>MAMGQLQHGIDDENATKQTQKYRDAEQSKKTAYDQAVAAAKAILNKQTGSNSDKAAVDRALQQVTSTKDALNGDAKLAEAKAAARQNLGTLNHITNAQRTALEGQINQATTVDGVNTVKTNANTLDGAMNSLQGAINDKDATLRNQNYLDADESKRNAYTQAVTAAEGILNKQTGGNTSKADVDNAL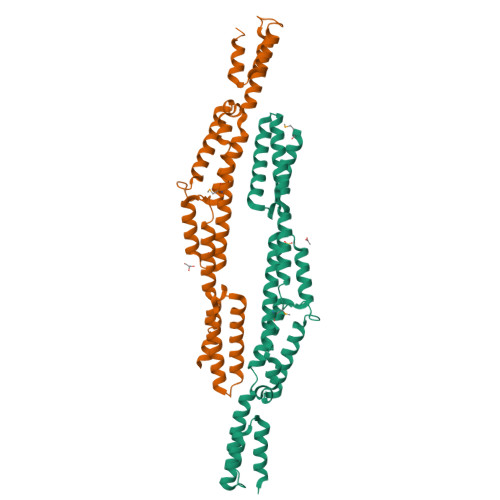NAVTRAKAALNGAENLRNAKTSATNTINGLPNLTQLQKDNLKHQVEQAQNVVGVNGVKDKGNLEHHHHHH[2x]>SMRTVEVTLHKEGNTFGFVIRGGAHDDRNKSRPVVITSVRPGGPADREGTIKPGDRLLSVDG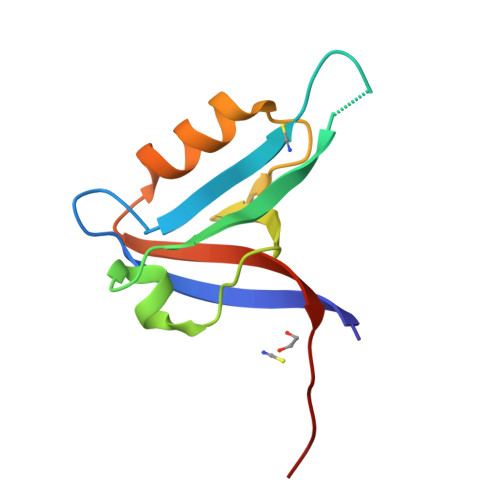IRLLGTTHAEAMSILKQCGQEAALLIEYDVSETAV[2x]>MADQQTTMPRWVPLLLGLLGSTTCGMLLYAWSVFIKPLNAEFGWSRAEIAMAFAICCLIFGLMTFPAGRLSDKMGPRKVVMTGGVLLAIGFILSGFIQSKYQLYITYGVIAGFGGGMIYLPPIATAPKWWPDRRALATGFAVVGLGLGSFLMGPLATYIIEKPGMGWRYVFWYCGVAMGIMALIAGAFLEPPPAGWKPAGYTPPAPPAGAAAPKVTRDWTYEEAKGDTKFWLLYLAYFCGSFAGLMVIGHLAGFGRDAGLTAMAAAGAVSSLAFSNAATRILSGWFVDKIGIRVYFAA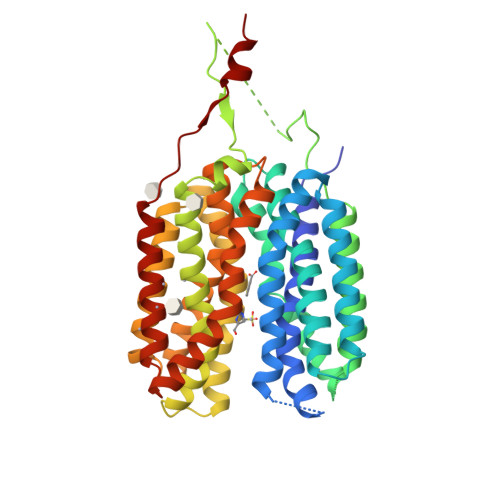LFALQTAAMIAIFQLGGSVVGLSIVAIVIGWNYGAMFTLFPATCLQFYGPTAQGSNYGLLFTACGLAGFAGPWVGGWLKDTTGTYYLPFLCAAALCALGTAIVFMTKPPEKKHALELEVLFQ[2x]> MQDVRVQVLPEVRGQLGGTVELPCHLLPPVPGLYISLVTWQRPDAPANHQNVAAFHPKSGPSFSSPKPGSERLSFVSAKQSTGQDTEAELQDATLALHGLTVEDEGNYTCE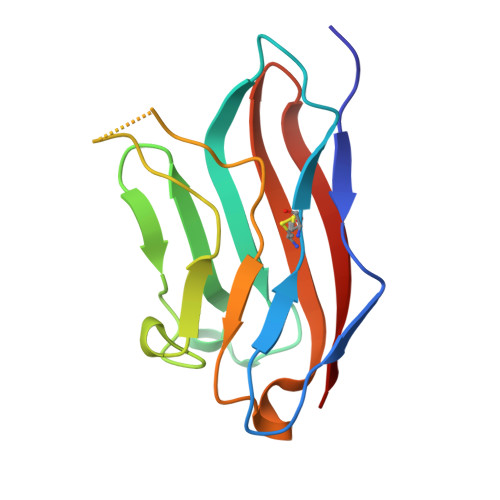FSTSPKGSVRGMTWLRV> MSLFDKKHLVSPADALPGRNTPMPVATLHAVNGHSMTNVPDGMEIAIFAMGAFWGVERLFWQLPGVYSTAAGYTGGYTPNPTYREVASGDTGHAEAVRIVYDP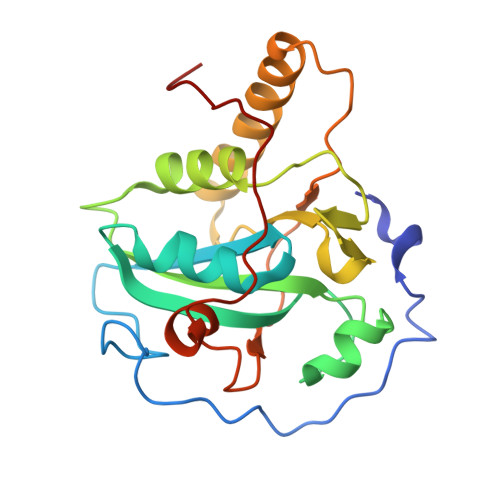SVISYEQLLQVFWENHDPAQGMRQGNDHGTQYRSAIYPLTPEQDAAARASLERFQAAMLAADDDRHITTEIANATPFYYAEDDHQQYLHKNPYGYAGIGGIGVCLPPEA>ASNFTQFVLVDNGGTGDVTVAPSNFANGVAEWISSNSRSQAYKVTASVRQSSAQNRKYTIKVEVPKVATVTVGGVELPVAAWRSYLNMELTIPIFAT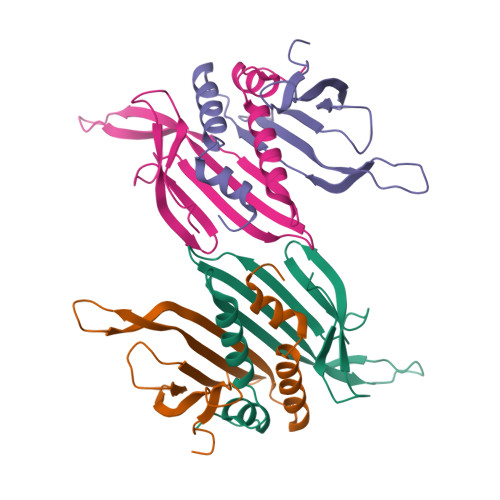NSDCELIVKAMQGLLKDGNPIPSAIAANSGIY[4x]>TYCVAMHLADGLVFASDSRTNAGIDHIATFRKLFTFGTPGERLLVVQTAGNLATSQSVINLLQQRIRRDGASLLNVPSVYDATALVAETTREVMARDSGNLAGNTDLSCSFMVGGQIAGGPPALYSIYPQGNFIQATPDTPFLQLGESKYGKPI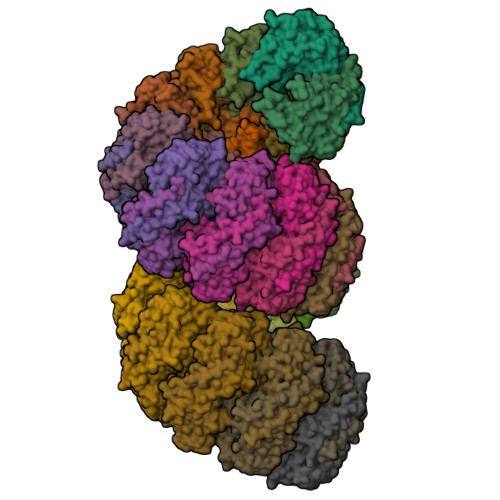LDRNLTFDTPLEQALRCALVSFDSTIRSNLSVGMPLDLLVYHRDSLILPEGYRVTEDDAYFSAIRRQWSAGLHDMLERLPSPPSAYNI[34x]> MIKEMIEDFISKGGLIFTHSGRYTNTNNSCFIFNKNDIGVDTKVDMYTPKSAGIKNEEGENLWQVLNKAN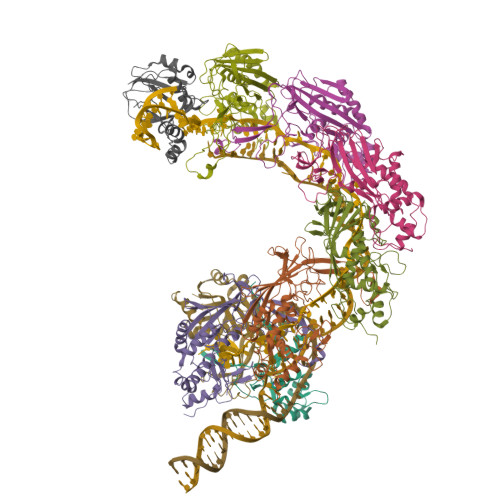MFYRIYSGELGEELQYLLKSCCTAKEDVTTLPQIYFKNGEGYDILVPIGNAHNLISGTEYLWEHKYYNTFTQKLGGSNPQNCTHACNKMRGGFKQFNCTPPQVEDNYNA;> MRKFIIVKNVKVDGINAKSSDITVGMPPATTFCGLGETMSIKTGIVVKAVSYGSVKFEVRGSRFNTSVTKFAWQDRGNGGKANNNSPIQPKPLADGVFTLCFEVEWEDCAEVLVDKVTNFINTARIAGGTIASFNKPFVKVAKDAEELASVKNAMMPCYVVVDCGVEVNIFEDAVNRKLQPMVNGYKKLEKIVDNKHMRDKFTPAYLATPTYTMIGYKMVSNVDNFDQALWQYGENTKVKTIGGIYND;>[6x]MTKLKAPAVLAYSRKINPTNALMFAVNWSDRDNTTAVMVGTKTVAGTQSVRGNPNDADKGNIQTVNFANLPHNKNTLLVKYNVKFVGDVFKAELGGGEYSNTLQTALENTDFGTLAYRYVYNIAAGRTLWRNRVGAESIETVITVNDQTFTFSDLLVNEFDEDVDVAEIADMVAGVLSGEGFVTLKVEHYMLLGEGSEVFPSQEFVENSKLSKQLFDLNGQAAMHDQKIGNAIRTIDTWYEDATTPIAVEPYGSVVRNGVAYRAGNKTDLFTLMDGAVNGKSLTEEDQMFVTANLIRGGVFGGGKD;> MYNTISITVVDADDVGVNFVVSKVLSTLHNKGIFNGEVGVTFPRMDKNVGDIITLFSKTGVDRKVLTSTLNTLTDFIHIGKPKEADKVKTYRKVDTKSKGKLIRRCIKRKGVSAETAESLYGNYKGEKCKLPYIVVNSKSTGQRFSMFLEECENSEKFNSYGLCIVSC> AWDYDNNVIRGVNLGGWFVLEPYMTPSLFEPFQNGNDQSGVPVDEYHWTQTLGKEAALRILQKHWSTWITEQDFKQISNLGLNFVRIPI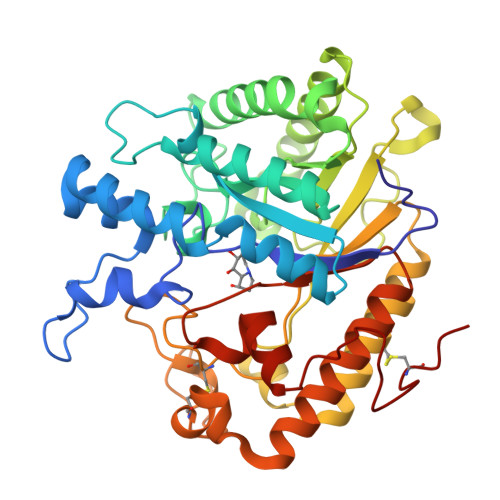GYWAFQLLDNDPYVQGQVQYLEKALGWARKNNIRVWIDLHGAPGSQNGFDNSGLRDSYNFQNGDNTQVTLNVLNTIFKKYGGNEYSDVVIGIELLNEPLGPVLNMDKLKQFFLDGYNSLRQTGSVTPVIIHDAFQVFGYWNNFLTVAEGQWNVVVDHHHYQVFSGGELSRNINDHISVACNWGWDAKKESHWNVAGEWSAALTDCAKWLNGVNRGARYEGAYDNAPYIGSCQPLLDISQWSDEHKTDTRRYIEAQLDAFEYTGGWVFWSWKTENAPEWSFQTLTYNGLFPQPVTDRQFPNQCGFH> LH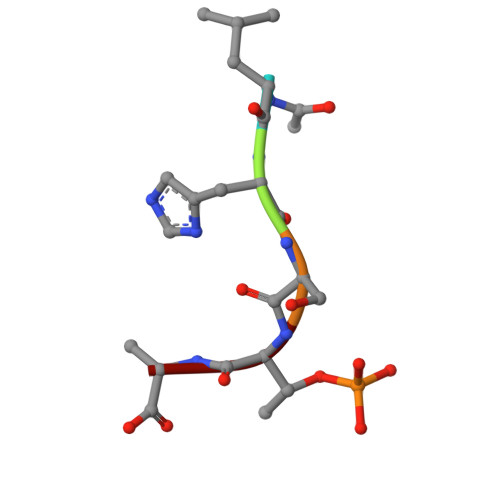STA> EWVKFAKPCREGEDNS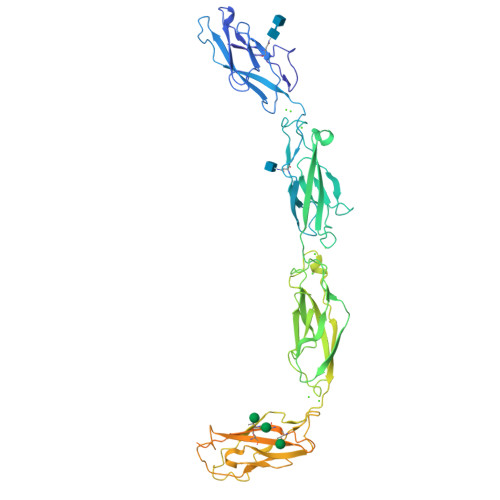KRNPIAKITSDYQATQKITYRISGVGIDQPPFGIFVVDKNTGDINITAIVDREETPSFLITCRALNAQGLDVEKPLILTVKILDINDNPPVFSQQIFMGEIEENSASNSLVMILNATDADEPNHLNSKIAFKIVSQEPAGTPMFLLSRNTGEVRTLTNSLDREQASSYRLVVSGADKDGEGLSTQCECNIKVKDVNDNFPMFRDSQYSARIEENILSSELLRFQVTDLDEEYTDNWLAVYFFTSGNEGNWFEIQTDPRTNEGILKVVKALDYEQLQSVKLSIAVKNKAEFHQSVISRYRVQSTPVTIQVINVREGIAFRPASKTFTVQKGISSKKLVDYILGTYQAIDEDTNKAASNVKYVMGRNDGGYLMIDSKTAEIKFVKNMNRDSTFIVNKTITAEVLAIDEYTGKTSTGTVYVRVPDFNDNCPTAVLEKDAVCSSSPSVVVSARTLNNRYTGPYTFALEDQPVKLPAVWSITTLNATSALLRAQEQIPPGVYHISLVLTDSQNNRCEMPRSLTLEVCQCDNRGICGTSHHHHHH> SGGAMHGDSLVQLSDSSFKMVKEVKKGDKVICPLLENQCVEVEC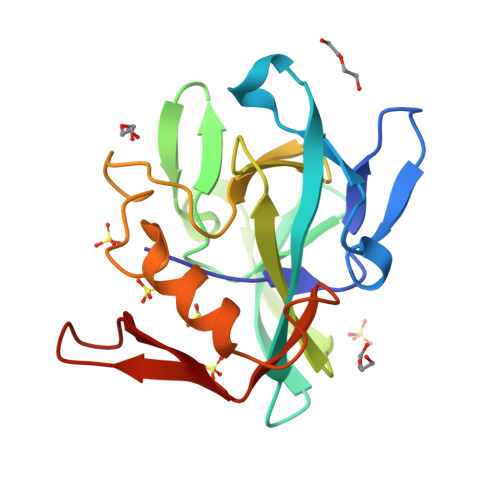VVLSKCEDGTKEFVQLGTDLWITPKHPIRVNGEWKYPKELGQTVVKTSDYIYQFVLKTGHTMNIGGYECICLGHNFQERVAYHPYLGSQAVVEDLKQMKGWKEGKVIIRSRVRDQITNQVKAFIQ>MNLLRRSGKRRRSESGSDSFSGSGGDSSASPQFLSGSVLSPPPGLGRCLKAAAAGECKPTVPDYERDKLLLANWGLPKAVLEKYHS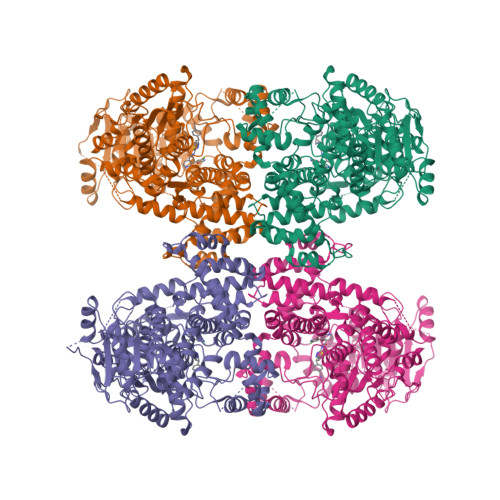FGVKKMFEWQAECLLLGQVLEGKNLVYSAPTSAGKTLVAELLILKRVLEMRKKALFILPFVSVAKEKKYYLQSLFQEVGIKVDGYMGSTSPSRHFSSLDIAVCTIERANGLINRLIEENKMDLLGMVVVDELHMLGDSHRGYLLELLLTKICYITRKSASCQADLASSLSNAVQIVGMSATLPNLELVASWLNAELYHTDFRPVPLLESVKVGNSIYDSSMKLVREFEPMLQVKGDEDHVVSLCYETICDNHSVLLFCPSKKWCEKLADIIAREFYNLHHQAEGLVKPSECPPVILEQKELLEVMDQLRRLPSGLDSVLQKTVPWGVAFHHAGLTFEERDIIEGAFRQGLIRVLAATSTLSSGVNLPARRVIIRTPIFGGRPLDILTYKQMVGRAGRKGVDTVGESILICKNSEKSKGIALLQGSLKPVRSCLQRREGEEVTGSMIRAILEIIVGGVASTSQDMHTYAACTFLAASMKEGKQGIQRNQESVQLGAIEACVMWLLENEFIQSTEASDGTEGKVYHPTHLGSATLSSSLSPADTLDIFADLQRAMKGFVLENDLHILYLVTPMFEDWTTIDWYRFFCLWEKLPTSMKRVAELVGVEEGFLARCVKGKVVARTERQHRQMAIHKRFFTSLVLLDLISEVPLREINQKYGCNRGQIQSLQQSAAVYAGMITVFSNRLGWHNMELLLSQFQKRLTFGIQRELCDLVRVSLLNAQRARVLYASGFHTVADLARANIVEVEVILKNAVPFKSARKAVDEEEEAVEERRNMRTIWVTGRKGLTEREAAALIVEEARMILQQDLVEMGVQWNPCALL[4x]>MNIRERKRKHLEACLEGEVAYQKTTTGLEGFRLRYQALAGLALSEVDLTTPFLGKTLKAPFLIGAMTGGEENGERINLALAEAAEALGVGMMLGSGRILLERPEALRSFRVRKVAPKALLIANLGLAQLRRYGRDDLL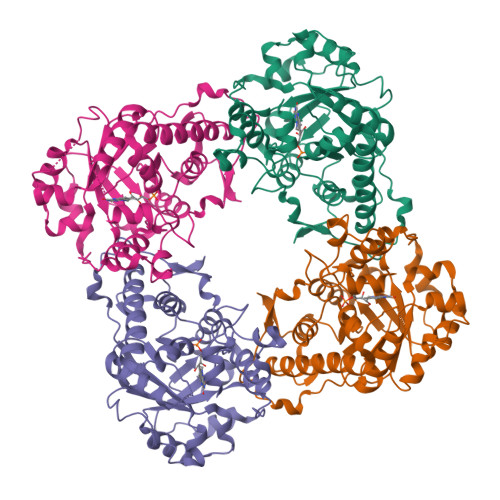RLVEMLEADALAFHVNPLQEAVQRGDTDFRGLVERLAELLPLPFPVMVKEVGHGLSREAALALRDLPLAAVDVAGAGGTSWARVEEWVRFGEVRHPELCEIGIPTARAILEVREVLPHLPLVASGGVYTGTDGAKALALGADLLAVARPLLRPALEGAERVAAWIGDYLEELRTALFAIGARNPKEARGRVERV[4x]>[4x]MGSDKIHHHHHHENLYFQGMKLGVNLCFAVKRWLEPDRLAGLVRDDLGLEYVQYTYDLTDPWWPDIERDRRAIAYAKAFRKAGLTIESTFGGLASYTYNHFLAPTLELQSLGYQHLKRAIDMTAAMEVPATGMPFGSYSAADALNPARREEIYAIARDMWIELAAYAKRQGLSMLYVEPVPLATEFPS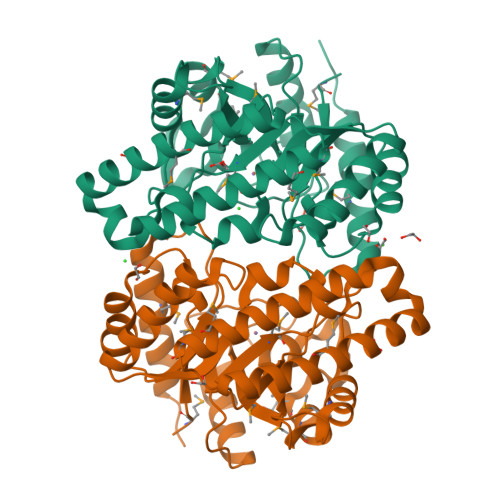SAADAARLMADLDGRTEIPVRLLVDWGHALFEPLFGPEADMDHWMDLCQPWIAAYHIQQTDGQLDRHWSFTQPGVVTPQRLQDFWDKYALTDQTFFAEILYPFEARDEDVLADMIASVKALKAASPAA>[2x]GGHMKWLIFGNKGWIGSMVSKILEQQGEQVVGAQSRADDESAVEREISE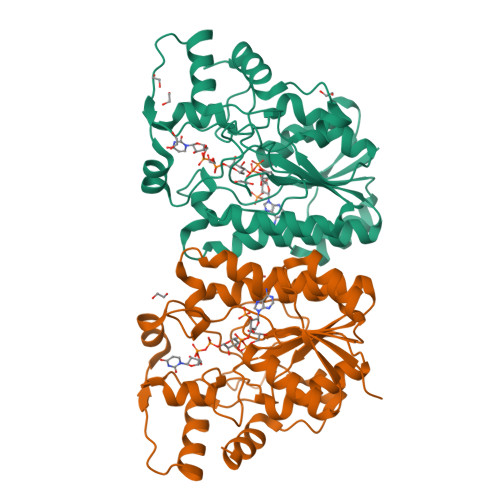IKPDRVMSFIGRTHGPGYSTIDYLEQSGKLVENVKDNLYGPLCLAFICQKYNIHLTYLGTGCIFEGQNNFSADEKGFTENDKPNFFGSSYSVVKGFTDRLMHFFDNDVLNLRIRMPITIEQNPRSFITKILSYSRICSIPNSMTILDQMIPVMIDMARNKTTGTFNFTNPGLVSHNEILSLIRDIHKPNLTWENMSREQQLAILKADRSNNLLNTDKLQSLYPDVPDILTGIREVVSKMKFQQ> GPHMSTFIFPGDSFPVDPTTPVKLGPGIYCDPNTQEIRPVNTGVLHVSAKGK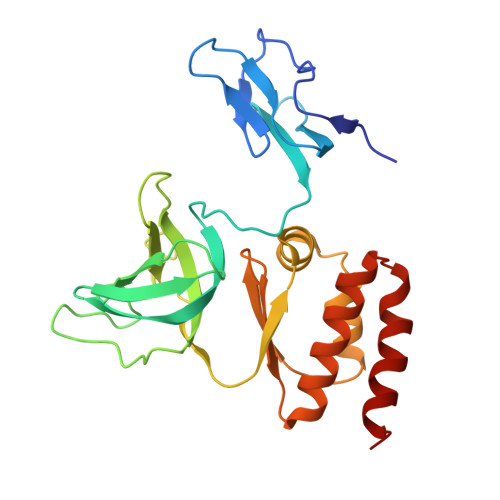SGVQTAYIDYSSKRYIPSVNDFVIGVIIGTFSDSYKVSLQNFSSSVSLSYMAFPNASKKNRPTLQVGDLVYARVCTAEKELEAEIECFDSTTGRDAGFGILEDGMIIDVNLNFARQLLFNNDFPLLKVLAAHTKFEVAIGLNGKIWVKCEELSNTLACYRTIMECCQKNDTAAFKDIAKRQFKEILTVKEE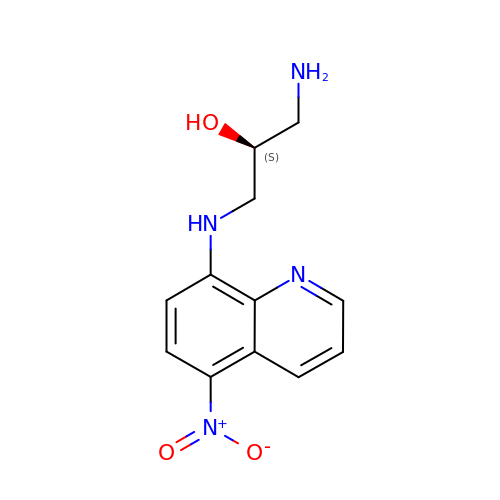(2S)-1-AMINO-3-[(5-NITROQUINOLIN-8-YL)AMINO]PROPAN-2-OL | C12 H14 N4 O3 | MBZPCTWLFNYBND-QMMMGPOBSA-N> MNKKQNFYAAIIVAIFLCLQLSHGSSGVSFEKTPAIKIVGNKFFDSESGEQFFIKGIAYQLQRSEEELSNANGAFETSYIDALADPKICLRDIPFLKMLGVNTLRVYAIDPTKSHDICMEALSAEGMYVLLDLSEPDISINRENPSWDVHIFERYKSVIDAMSSFPNLLGYFAGNQVTNDHTNTFASPFVKAAIRDAKEYISHSNHRKIPVGYSTNDDAMTRDNLARYFVCGDVKADFYGINMYEWCGYSTYGTSGYRERTKEFEGYPIPVFFSEFGCNLVRPRPFTEVSALYGNKMSSVWSGGLAYMYFEEENEYGVVKINDNDGVDILPDFKNLKKEFAKADPKGITEEEYLTAKEPTEVESVECPHIAVGVWEANEKLPETPDRSKCACLDEILPCEIVPFGAESGKYEEYFSYLCSKVDCSDILANGKTGEYGEFSDCSVEQKLSLQLSKLYCKIGANDRHCPLNDKNVYFNLESLQPLTSESIC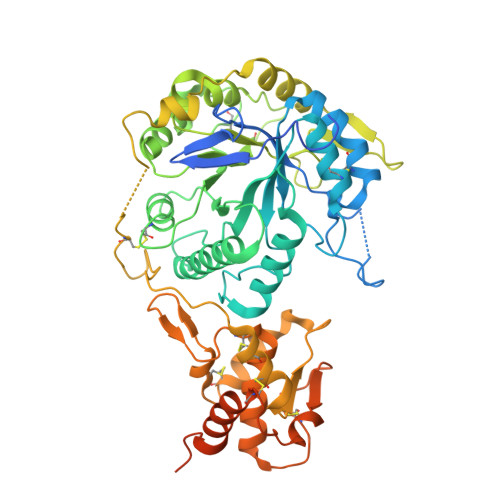KNVFDSIRNITYNHGDYSKSNPSRSKESLNVKYPSSEERENDGTIAFKTSGFVILLISMIAAGILL> DLTKNEKGRLTPITKQQSANSAKLTAYGTLKSALEKFQTANTALNKADLFKSTVASSTTEDLKVSTTAGAAAGTYKINVTQLAAAQSLATKTTFATTKEQLGDTSVTSRTIKIEQPGRKEPLEIKLDKGDTSMEAIRDAINDADSGIAASIVKVKENEFQLVLTANSGTDNTMKITVEGDTKLNDLLAYDSTTNTGNMQELVKAENAKLNVN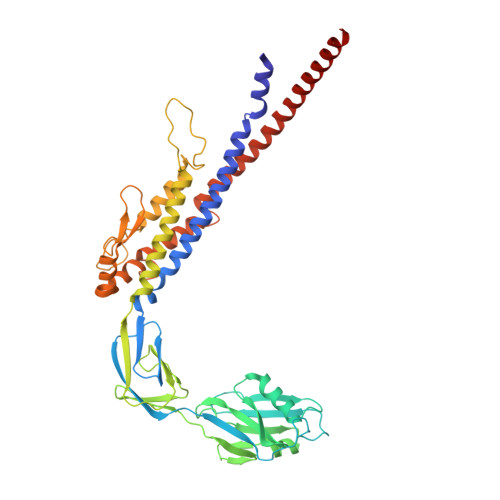GIDIERQSNTVTDAPQGITLTLTKKVTDATVTVTKDDTKAKEAIKSWVDAYNSLVDTFSSLTKYTAVEPGEEASDKNGALLGDSVVRTIQTGIRAQFANSGSNSAFKTMAEIGITQDGTSGKLKIDDDKLTKVLKDNTAAARELLVGDGKETGITTKIATEVKSYLADDGIIDNAQDNVNATLKSLTKQYLSVSNSIDETVARYKAQFTQLDTMMSKL> MIQEHRYDVVIVGAGGAGMRAAVEAGPRARTAVLTKLYPTRSHTGAAQGGMCAALANVEEDNWEWHTFDTVKGGDYLADQDAVEIMCKEAIDAVLDLEKMGMPFNRTPEGRIDQRRFGGHTRDHGKAPVRRACYAADRTGHMILQTLYQNCVKHDVEFFNEFYALDIALTETPAGPVATGVIAYELATGDIHVFHAKAIVFATGGSGRMYKTTSNAHTLTGDGLGIVFRKGLPLEDMEFHQFHPTGLAGLGILISEAVRGEGGRLLNGEGERFMERYAPTIVDLAPRDIVARSMVLEVLEGRGAGPNKDYVYIDVRHLGEDVLEAKLPDITEFARTYLGVDPVKELVPVYPTCHYVMGGIPTTVNGQVLRDNTNVIPGLYAAGECACVSVHGANRLGTNSLLDIN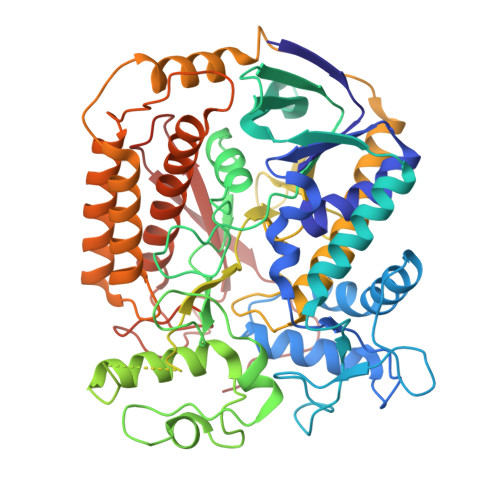VFGRRAGIAAAEYAQNHNFVDMPENPAEMVVGWVGDILSEHGNERVADIRGALQQSMDNNAAVFRTEETLKQALTDIHALKERYSRITVHDKGKRYNSDLLEAIELGFLLELAEVTVVGALNRKESRGGHAREDYPNRDDTNYMRHTMAYKQGTDLLSDIRLDYKPVVQTRYEPMERKY> MTFAKIKFSAQIRLETGLHIGGSDAFAAIGAIDSPVIKDPITNIPIIPGSSLKGKMRTLLAKVYNEKVAEKPSD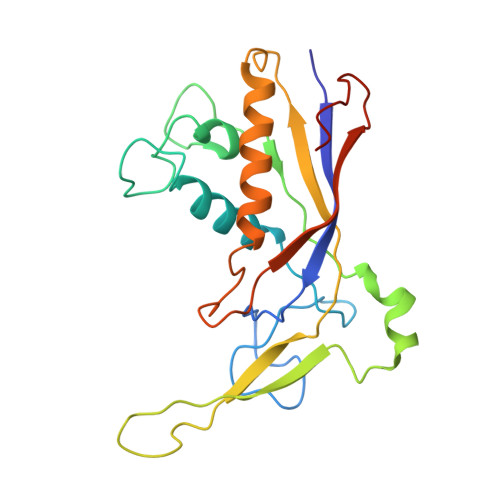DSDILSRLFGNSKDKRFKMGRLIFRDAFLSNADELDSLGVRSYTEVKFENTIDRITAEANPRQIERAIRNSTFDFELIYEITDENENQVEEDFKVIRDGLKLLELDYLGGSGSRGYGKVAFEKLKATTVFGNYDVKTLNELLTAEV>MKKYTCTVCGYIYNPEDGDPDNGVNPGTDFKDIPDDWVCPL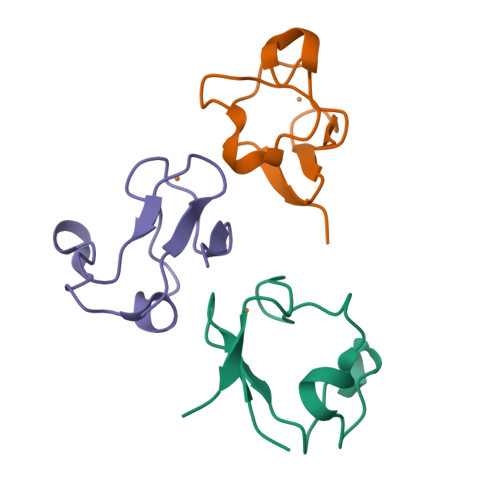CGAGKDQFEEVEE[3x]> MHHHHHHHHHHGENLTFQGMKKYKKFCFLGIGLLPLVLASCGTNTATKDSQDATEKKVEQVATLTAGTPVQSLDPATAVDQTSITLLANVMEGLYRLDEKNQPQPAIAAGQPKVSNNGKTYTIVIRDGAKWSDGTQITASDFVAAWQRVVDPKTVSPNVELFSAIKNAKEIASGKQAKDTLAVKSIGEKTLEIELVEPTPYFTDLLSLTAYYPVQQKAIKEYGKDYGVSQKAIVTNGAFNLTNLEGVGTSDKWTISKNKEYWDQKDVSMDKINFQVVKEINTGINLYNDGQLD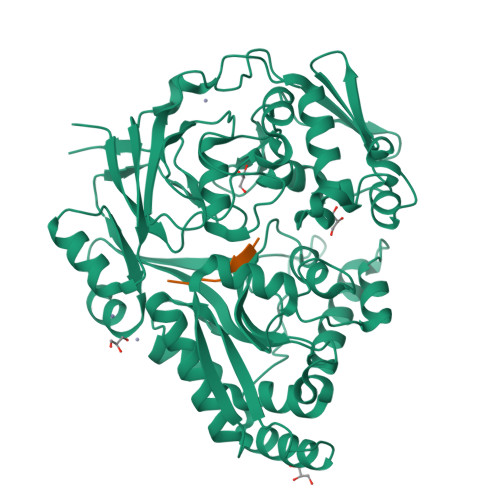EAPLAGEYAKQYKKDKEYSTTLMANTMFLEMNQTGENKLLQNKNVRKAINYAIDRESLVKKLLDNGSVASVGVVPKEMAFNPVNKKDFANEKLVEFNKKQAEEYWDKAKKEIDLSKNTSLDLLVSDGEFEKKAGEFLQGQLQDSLEGLKVTVTPIPANVFMERLTKKDFTLSLSGWQADYADPISFLANFETNSPMNHGGYSNKNYDELLKDSSSKRWQELKKAEKLLINDMGVVPIFQVGTAKLEKSKIKNVLMHSIGAKYDYKKMRIEK;> LVTLVFV methyl 7-fluoro-3-{4-[(2-hydroxyethyl)sulfonyl]benzyl}-4-oxo-1-phenyl-1,4-dihydroquinoline-2-carboxylate 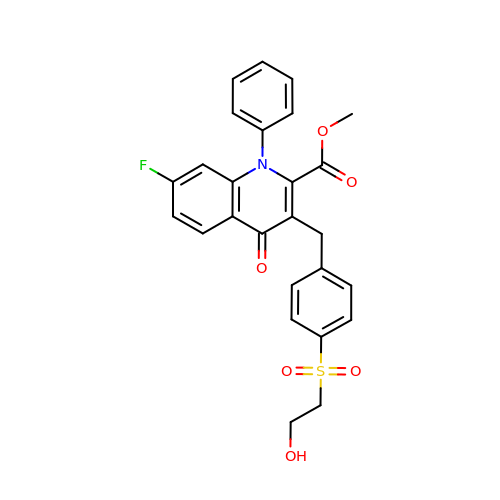| C26 H22 F N O6 S | RWVFVOHUWIBKDI-UHFFFAOYSA-N> MHHHHHHANIDESKIKDTVDDLIQPLMQKNNIPGMSVAVTVNGKNYIYNYGLAAKQPQQPVTENTLFEVGSLSKTFAATLASYAQVSGKLSLDQSVSHYVPELRGSSFDHVSVLNVGTHTSGLQLFMPEDIKNTTQLMAYLKAWKPADAAGTHRVYSNIGTGLLGMIAAKSLGVSYEDAIEKTLLPQLGMHHSYLKVPADQMENYAWGYNKKDEPVHVNMEILGNEAYGIKTTSSDLLRYVQANMGQLKLDANAKMQQALTATHTGYFKSGEITQDLMWEQ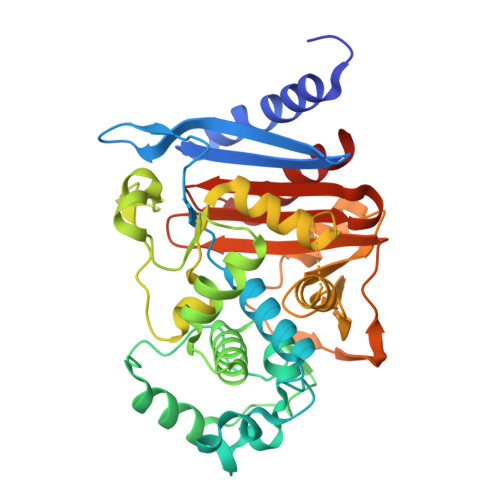LPYPVSLPNLLTGNDMAMTKSVATPIVPPLPPQENVWINKTGSTNGFGAYIAFVPAKKMGIVMLANKNYSIDQRVTVAYKILSSLEGNK> MSDNTMNTEEIENENGFDIINDFNKVLKYNEISLKSFSDHSSNQWREFTIDSNSQGYYGYSNNNDINFIQDKFTSTPYRSGGFNYKKSPLTDGRFIIWRLVNKSSTLELCEHYSHHSLESNQIRIHFNNTSIIGDVFIQELNDYVIIMVTTISKTIYRFLLPHPSIIEHSDSRVGIKRKVEVDSFGSGSGNNNKRNYKSIFSNLLNSNLDNQWSRVRGVLPDSFEPTVIRYYSATKLIIGSSGSGSTWLELSDIKQSGDITVKKFDCKEGQGFFSSWKWGEKQEPVQDIQFLSTTTNSNNNNNFPLALILLNNSQLKVWSANDKKFIKEITISPENWNNNNNNNNENNNNNNNNIPTSPNINSNQQQQQQQNLSLIHKRFKIYQRSTKSFLLVVYFQFNSESQFQFFSGTNDFSNGINIKEERFAFLKGKGLIDFNIHNGILYSIWSQIKERNYNRGRINRDQEFDEDDNKFDRNHFVDDNNDQEEEVIFKHIYIGDLINFNHQKLSTSNGNGNGNGNNNLENEKEINMEYNQFYNGEMINTFDKYYETIIEHSDEDSDQPTDQTYYYNLLFNRGLFSPNSIEQALNEYKKLKDIDDHGGDNDVEMNNGFDNDNSLESVVSNILNQEDFKFQSNEQWSIFFKLCTKFQKQTCLLGSGLFIEPTSSIIFLIRSNQLSIMKPMKPIECLYTISNNINNSNIISDKQFYNIILNCFGSNSNVLVNDFLYLMKCCNFIDRFIKDDYRSFEYELSRQHVNHTLLKVSEKLIANSYNNSNNNNNNNNNSNNNNIEDNINNYSIGFIKLFKLIENPIETINLILKKFKEEFSNQNDMVIQLQQGYKNIDKGWSGDLFADILTNCFVSTIEIKYQLLTKLSLLLGTVSNLRTHLGIDTKTLFTLEKSILPDSIKLLSTYYLLNWFTKQNFIKSFDNSTTSDIDKILISQNQYGDDSDNNNNINNNEYYEDQQQQQNQQQFTISKNLNILTILINRNLNQFTSKNEFFENIEKQLSKLLCVLAPHMDLFSMGCYLVEKNQYKQLMEFLQIIENNELIEMITPFYYLMGICYAHYSKFNEAYQYLLKATESIENQNQDM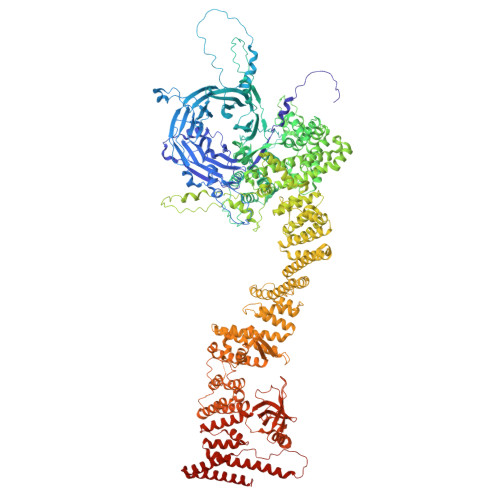LKICSISKEELVCSLFVDIPIDNRMMNQTNANTTQTLISNYYLKCIKIFETRNQPEFIIQFSLFAIDYLTLEKENFSRLDYLNKLESLYSLVFKYSLKIQEYDLAFTASTLNPNQDVSQENKRRLILTLCENSVTTVNNNNNNNNNNNTNNNTNNNNNIGSGNSIKVLCKLPFPQKDIEDNLLKLASAQDLNKKPDYHTILYAYYISRCNYRNASMIYYERSIRVNIEGLGKSRGKSIFDQQQLLDTKLELLSTTINTLKLLDPSDQWIEINSSSLDIRSTNIYNNNSSLNIANHHQHQHQQRKFNYIGNNDEFKDISVVTLKEIEKEYSYYLASKHLCSIDSQINSDFILSPQQLLEKLIQYSLFDVAFSLAITQEIDLGAIFESFASKCVQLQLNPQSNPFFIKNTNGYGSGVIGNGANNNNNNYGFDCSELQHLKDKVTLTWKVLENYLQRYDSDKDFQCLSPSEINENSQNPNTKATIIGNQQMQLRMFGEIQQGSLVDRDCNGCSFRVSDSKGFYLDVHYSHRVPPFFNDTQSGQQVIVIGKLQDGRFIADNVLCKQGQLRYHELVADTILYEGTLDLPTWLIQWFSKGRQDTLFKLYFRHSRLIDASITLRDLFKHAQFELNQINNNNNNNNTIKTSSQITSKTISLNIPYDLIDRFFIEAKKIKSSIIDQKEKQQLTQELTLAENEMIKYFSKVN> MSNMEKHLFNLKFAAKELSRSAKKCDKEEKAEKAKIEKAIQKGNMEVARIHAENAIRQKNQAVNFLRMSARVDAVAARVQTAVTMGKVTKSMAGVVKSMDATLKTMNLEKISALMDKFEHQFETLDVQTQQMEDTMSSTTTLTTPQNQVDMLLQEMADEAGLDLNMELPQGQTGSVGTSVASAEQDELSQR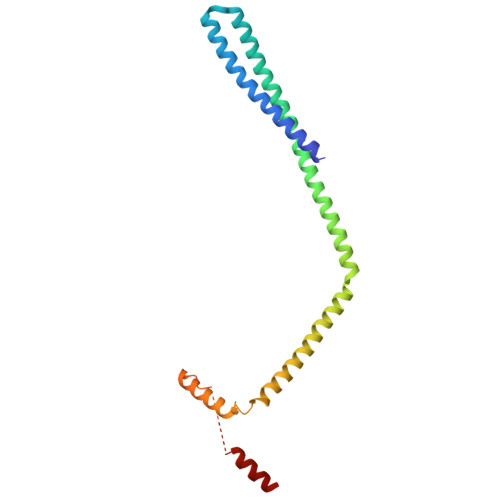LARLRDQV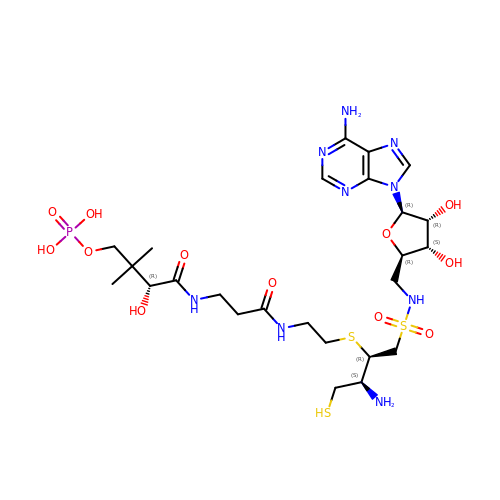5'-{[(2R,3S)-3-amino-2-({2-[(N-{(2R)-4-[(dihydroxyphosphanyl)oxy]-2-hydroxy-3,3-dimethylbutanoyl}-beta-alanyl)amino]ethyl}sulfanyl)-4-sulfanylbutane-1-sulfonyl]amino}-5'-deoxyadenosine | C25 H44 N9 O12 P S3 | DMSHVJWQIKPFOK-DROAMXOMSA-N> MILDADYITEDGKPIIRIFKKENGEFKVEYDRNFRPYIYALLKDDSAIEDVKKITAERHGTTVRVVRAEKVKKKFLGRPI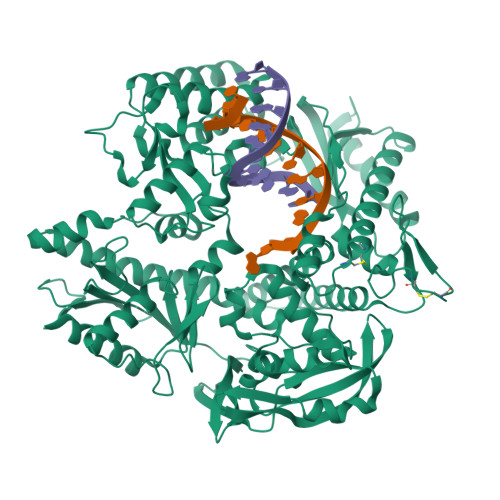EVWKLYFNHPQDQPAIRDRIRAHPAVVDIYEYDIPFAKRYLIDKGLIPMEGDEELTMLAFAIATLYHEGEEFGTGPILMISYADGSEARVITWKKIDLPYVDVVSTEKEMIKRFLRVVREKDPDVLITYNGDNFDFAYLKKRCEELGIKFTLGRDGSEPKIQRMGDRFAVEVKGRIHFDLYPVIRRTINLPTYTLEAVYEAIFGQPKEKVYAEEIAQAWETGEGLERVARYSMEDAKVTYELGKEFLPMEAQLSRLIGQSLWDVSRSSTGNLVEWFLLRKAYERNELAPNKPDEREYERRLRESYAGGYVKEPEKGLWEGLVSLDFRSLGPSIIITHNVSPDTLNREGCREYDVAPEVGHKFCKDFPGFIPSLLGDLLEERQKVKKKMKATIDPIEKKLLDYRQRLIKILANSFYGYYGYAKARWYCKECAESVTAWGRQYIETTIREIEEKFGFKVLYADTDGFFATIPGADAETVKKKAKEFLDYINAKLPGLLELEYEGFYKRGFFVTKKKYAVIDEEDKITTRGLEIVRRDWSEIAKETQARVLEAILKHGDVEEAVRIVKEVTEKLSKYEVPPEKLVIYKQITRDLKDYKATGPHVAVAKRLAARGVKIRPGTVISYIVLKGSGRIGDRAIPFDEFDPTKHKYDAEYYIENQVLPAVERILRASHYRKEDLRYQKTRQVGLSAWLKPKT>GSHMAIATINPTTGEICQRFKALTPAEIDAKLAKAQEAFQAYRRTSFSQRRQWLENAAAILERDTSKFAEIMTTEMGKTHQSAIAEAEKSALVCRYYAEHGEQFLANEYTETQATESYVCYQPLGILLAVMPWNFPFWQVFRFAAPALMAGNVAVLKHASNVPQCALAVEAILEAAGFPEGVFQTLLIGASQVEQVIKDPRVKAATLTGSEPAGASLASLAGQEIKPTLLELGGSDPFVVFPSADLDEAVEVGTVARTMNNGQSCIAAKRFILHEAIAAEFLEKLHLKFASLKIGDPMAPETDIGPLATEGILQDISRQVDQAVAAGAKILLGGRPLDRAG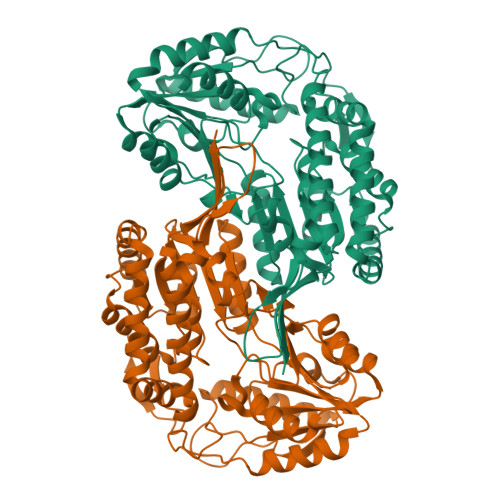YFYPPTILTEIPPGAKILQEELFAPVAMVFTVKDLDQAIALANDIPFGLGASAWTNDPAEQQRFIQELDAGAVFINGMVKSDPRLPFGGTKRSGYGRELGLAGIRTFVNAKTVWLK[2x]(3R)-4-[(3R)-3-AMINO-4-(2,4,5-TRIFLUOROPHENYL)BUTANOYL]-3-METHYL-1,4-DIAZEPAN-2-ONE | C16 H20 F3 N3 O2 | 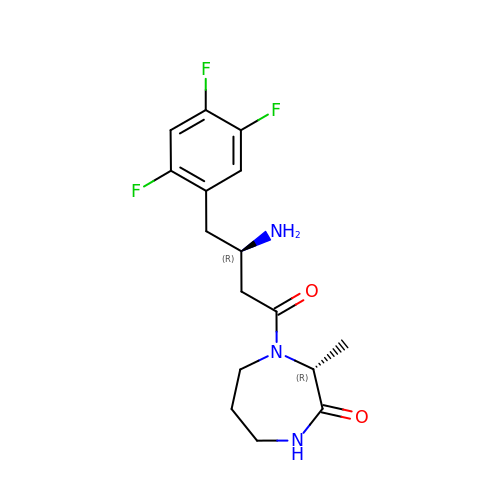SWKGZJAAGSVROJ-MWLCHTKSSA-N>[2x]INAGTDLDNPKDLEVSDPTETTLSLRWRRPVAKFDRYRLTYVSPSGKKNEMEIPVDSTSFILRGLDAGTEYT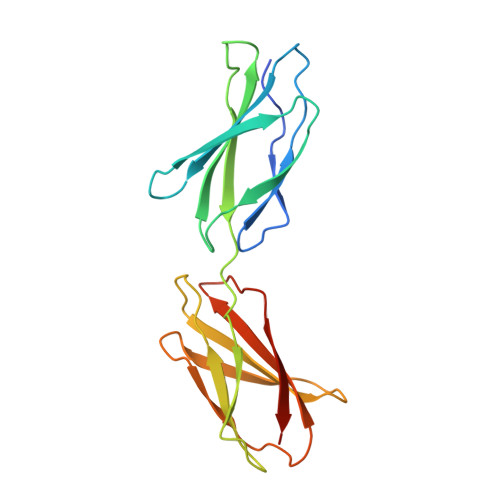ISLVAEKGRHKSKPTTIKGSTVVGSPKGISFSDITENSATVSWTPPRSRVDSYRVSYVPITGGTPNVVTVDGSKTRTKLVKLVPGVDYNVNIISVKGFEESEPISGILKTALDS>[12x]GAMGIGKSPTGIQGFDELTLGGLPTGRPSLVCGSAGCGKTLFASTFLINGVRDHGEPGVFVTFEERPEDIVNNVASLGFELDKLIEEEKIAIEHIAVDPSEVAEIGDYDLEGLFLRLELAIDTVGAKRVVLDTIESLFSAFSNPAILRAEIRRLFDWLKERGLTTVITAERGDGALTRQGLEEYVSDCVILLDHRVENQISTRRLRIVKYRGTAHGTNEYPFLIDTDGFSVLPVSALGLLHQVHEERIASGVPDLDAMMAGGGFFRGSSILVSGVAGAGKSSLAAHFAAAACARGERAMYFSFEEAADQAVRNMRSLGLDLGRWRDAGLLRFMATRPTFYSLEMHLAVILREVMRFEPSVVVLDPISAFTESGDRLEVQSMLLRIVDFLKNRGITGIFTHLAHSQNEATTDAGLEELMDGWVLMLNREVNGEFNRELYLLKARGMAHSNQVREFLMSDRGISLLPPHL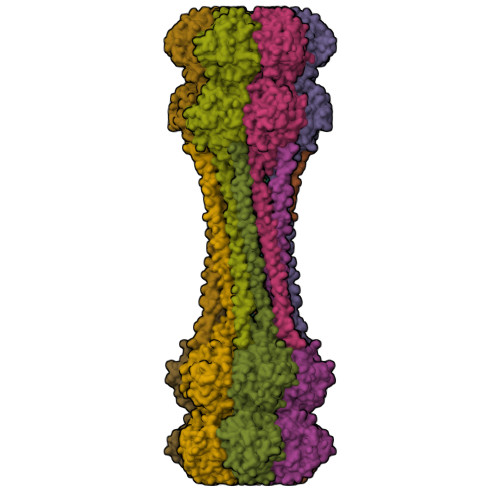GEGGALTGTARKAEEARLRRAEIERQTELGRLQQQIEQRRRRARAQIEALEAELQAEEIALKALVESESAHERQRLADADTLARSRGNERFADLLMNKGE>[4x]MLSRKGIIPEEYVLTRLAEDPAEPRYRTRERRARFVSKKGNCNVAHKNIREQGRFLQDVFTTLVDLKWPHTLLIFTMSFLCSWLLFAMVWWLIAFAHGDLAPGEGTNVPCVTSIHSFSSAFLFSIEVQVTIGFGGRMVTEECPLAILILIVQNIVGLMINAIMLGCIFMKTAQAHRRAETLIFSKHAVITLRHGRLCFMLRVGDLRKSMIISATIHMQVVRKTTSPEGEVVPLHQVDIPMENGVGGNGIFLVAPLIIYHVIDSNSPLYDLAPSDLHHHQDLEIIVILEGVVETTGITTQARTSYLADEILWGQRFVPIVAEEDGRYSVDYSKFGNTIKVPTPLCTARQLDEDRSLLDALTLASSRGPLRKRSVAVAKAKPKFSISPDSLS;>[4x]MPLAFCGTENHSAAYRVDQGVLNNGCFVDALNVVPHVFLLFITFPILFIGWGSQSSKVHIHHSTWLHFPGHNLRWILTFILLFVLVCEIAEGILSDGVTESRHLHLYMPAGMAFMAAITSVVYYHNIETSNFPKLLIALLIYWTLAFITKTIKFVKFYDHAIGFSQLRFCLTGLLVILYGMLLLVEVNVIRVRRYIFFKTPREVKPPEDLQDLGVRFLQPFVNLLSKGTYWWMNAFIKTAHKKPIDLRAIGKLPIAMRALTNYQRLCVAFDAQARKDTQSPQGARAIWRALCHAFGRRLILSSTFRILADLLGFAGPLCIFGIVDHLGKENHVFQPKTQFLGVYFVSSQEFLGNAYVLAVLLFLALLLQRTFLQASYYVAIETGINLRGAIQTKIYNKIMHLSTSNLSMGEMTAGQICNLVAIDTNQLMWFFFLCPNLWAMPVQIIVGVILLYYILGVSALIGAAVIILLAPVQYFVATKLSQAQRSTLEHSNERLKQTNEMLRGMKLLKLYAWESIFCSRVEVTRRKEMTSLRAFAVYTSISIFMNTAIPIAAVLITFVGHVSFFKESDLSPSVAFASLSLFHILVTPLFLLSSVVRSTVKALVSVQKLSEFLSSAEIREEQCAPREPAPQGQAGKYQAVPLKVVNRKRPAREEVRDLLGPLQRLAPSMDGDADNFCVQIIGGFFTWTPDGIPTLSNITIRIPRGQLTMIVGQVGCGKSSLLLATLGEMQKVSGAVFWNSNLPDSEGEDPSSPERETAAGSDIRSRGPVAYASQKPWLLNATVEENITFESPFNKQRYKMVIEACSLQPDIDILPHGDQTQIGERGINLSGGQRQRISVARALYQQTNVVFLDDPFSALDVHLSDHLMQAGILELLRDDKRTVVLVTHKLQYLPHADWIIAMKDGTIQREGTLKDFQRSECQLFEHWKTLMNRQDQELEKETVMERKASEPSQGLPRAMSSRDGLLLDEEEEEEEAAESEEDDNLSSVLHQRAKIPWRACTKYLSSAGILLLSLLVFSQLLKHMVLVAIDYWLAKWTDSALVLSPAARNCSLSQECDLDQSVYAMVFTLLCSLGIVLCLVTSVTVEWTGLKVAKRLHRSLLNRIILAPMRFFETTPLGSILNRFSSDCNTIDQHIPSTLECLSRSTLLCVSALTVISYVTPVFLVALLPLAVVCYFIQKYFRVASRDLQQLDDTTQLPLLSHFAETVEGLTTIRAFRYEARFQQKLLEYTDSNNIASLFLTAANRWLEVRMEYIGACVVLIAAATSISNSLHRELSAGLVGLGLTYALMVSNYLNWMVRNLADMEIQLGAVKRIHALLKTEAESYEGLLAPSLIPKNWPDQGKIQIQNLSVRYDSSLKPVLKHVNALISPGQKIGICGRTGSGKSSFSLAFFRMVDMFEGRIIIDGIDIAKLPLHTLRSRLSIILQDPVLFSGTIRFNLDPEKKCSDSTLWEALEIAQLKLVVKALPGGLDAIITEGGENFSQGQRQLFCLARAFVRKTSIFIMDEATASIDMATENILQKVVMTAFADRTVVTIAHRVHTILSADLVMVLKRGAILEFDKPETLLSQKDSVFASFVRADK

ATP-sensitive potassium channels (KATP) are ion channels that selectively allow potassium ions to permeate the cell. Specifically, they are inhibited by ATP and activated by Mg-ADP. Previous studies have established that the functional KATP channel is a hetero-octamer composed of four inward-rectifying potassium channel 6 (Kir6) subunits and four sulfonylurea receptor (SUR) regulatory subunits. KATP channels in pancreatic islets are composed of Kir6.2 channel subunits and SUR1 regulatory subunits.

The second structure is the KATP channel in complex with ATPγS alone, which is solved to 4.4 Å resolution (abbreviated, ATP state). Therefore, we applied ATPγS, a slowly hydrolyzable and functional ATP analog, to stabilize the structures of the KATP channel with and without GBM. The overall KATP channel structure and SUR1 conformation in the ATP + GBM state is almost identical to that in the ATP state based on our density maps. In contrast, this density is not present in the ATP state, where GBM was not supplied into the sample. Therefore, we compared the density maps around lasso motif between the ATP state and the ATP + GBM state, and found that the extra density near the lasso motif in the previous medium resolution map is present in both states. With improved resolution and map quality, we found that this extra density was contributed by both the M5-Lh1 loop and an unknown ligand, probably a lipid head group that constitutively binds KATP, because it is also present in the Mg-ADP state described later. We observed a similar density in the map of the ATP state structure. In the sample preparation procedure, we added 2 mmol/L ethylenediaminetetraacetic acid (EDTA) to avoid the activation effect of ATPγS by chelating divalent ions. Therefore, we observed an Mg-independent ATP binding site in the degenerate site on the NBD1 of SUR1. We observed ATP density only in the NBD1 degenerate site but not in the NBD2 consensus site, which suggests that the degenerate site has a higher affinity for Mg-free ATP, and ATP alone is not able to drive the dimerization of SUR1 NBDs.8-methoxy-4-methylquinolin-2(1H)-one | C11 H11 N O2 | 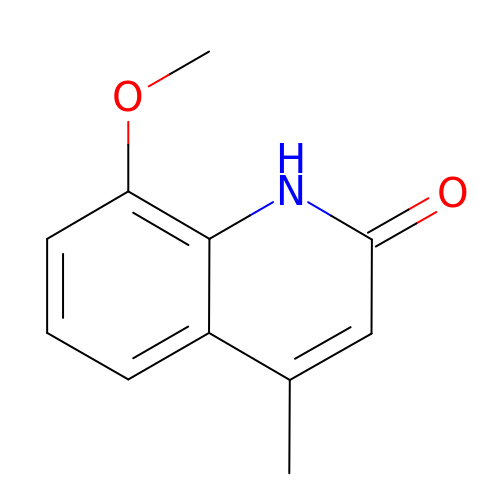WHZDFFGNQINQSU-UHFFFAOYSA-N> MRKIIVGSRRSKLALTQTKWVIEQLKKQGLPFEFEIKEMVTKGDQILNVTLSKVGGKGLFVKEIEQAMLDKEIDMAVHSMKNMPAVLPEGLTIGCIPLREDHRDALISKNGERFEELPSGAVIGTSSLRRGAQLLSMRSDIEIKWIRGNIDTRLEKLKNEDYDAIILAAAGLSRMGWSKDTVTQYLEPEISVPAVGQGALAIECRENDHELLSLLQALNHDETARAVRAERVFLKEMEGGCQVPIAGYGRILDGGNIELTSLVASPDGKTIYKEHITGKDPIAIGSEAAERLT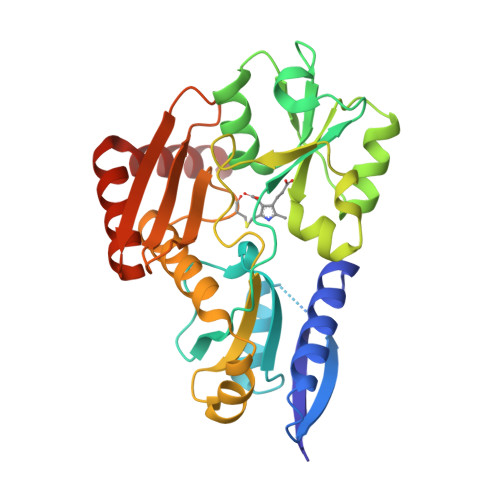SQGAKLLIDRVKEELDK> THFGILMD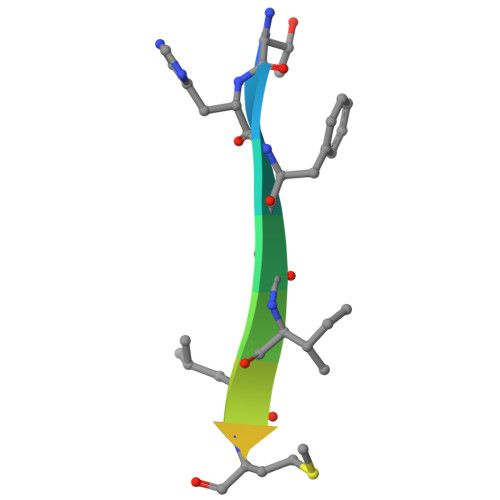VSRA Orsay, the only virus known to naturally infect the nematode Caenorhabditis elegans, expresses a capsid-δ fusion protein. We have demonstrated that the Orsay fusion protein is incorporated into Orsay capsid and forms a ~420-Å long fiber protruding from the capsid surface. Our model predicts that δ consists of three domains: an N-terminal helical domain that is covalently linked to the capsid, a middle shaft that is mostly β-stranded, and a C-terminal head that likely hosts the cell receptor binding site for host attachment. By analogy with other viral capsid-associated fiber proteins, the Orsay CP-δ likely functions in cell entry as a cell receptor binding protein.

Among these four constructs, only δ(1–66), which contains the first 66 residues of δ, produced crystals diffracted to better than 3-Å resolution. The structure of δ(1–66) was determined by single-wavelength anomalous dispersion (SAD) using SeMet-substituted crystals. By subsequent molecular replacement and refinement against a native dataset, we were able to establish the final structure to 2.2-Å resolution. δ(1–66) assembles into a pentamer with the five subunits forming an α-helical bundle. This five-helical bundle is ~80-Å long and ~35-Å wide. Each δ(1–66) molecule folds into two α-helices that are connected by a 9-aa linker (i.e. residues 21 to 29). The longer α-helix, consisting of residues 30 to 63, has a kink at around residue 40. The helix after the kink contains three regular heptad repeats (i.e. 40VSDKLDKISESLNTLVECVID60, in which hydrophobic residues are highlighted in bold). Surface representation of the δ(1–66) pentamer shows a ~3 to 5-Å wide channel running through the entire molecule. Therefore, the core of the entire helical bundle is mostly hydrophobic, except for a single location at T14.

>MPSEDYAIWYARATIAALQAAEYRLAMPSASYTAWFTDAVSDKLDKISESLNTLVECVIDKRLAVS[5x]>MTKPLILASQSPRRKELLDLLQLPYSIIVSEVEEKLNRNFSPEENVQWLAKQKAKAVADLHPHAIVIGADTMVCLDGECLGKPQDQEEAASMLRRLSGRSHSVITAVSIQAENHSETFYDKTEVAFWSLSEEEIWTYIETKEPMDKAGA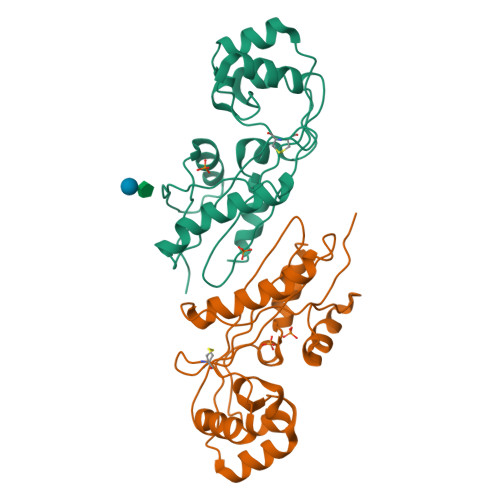YGIQGRGALFVKKIDGDYYSVMGLPISKTMRALRHFDIRA[2x]> HEDEIKKLRTSGSMTQNPHEVARVRNLNRIIMGKYEIEPWYFSPYPIELTDEDFIYIDDFTLQYFGSKKQYERYRKKCTLRHPPGNEIYRDDYVSFFEIDGRKQRTWCRNLCLLSKLFLDHKTLYYDVDPFLFYCMTRRDELGHHLVGYFSKEKESADGYNVACILTLPQYQR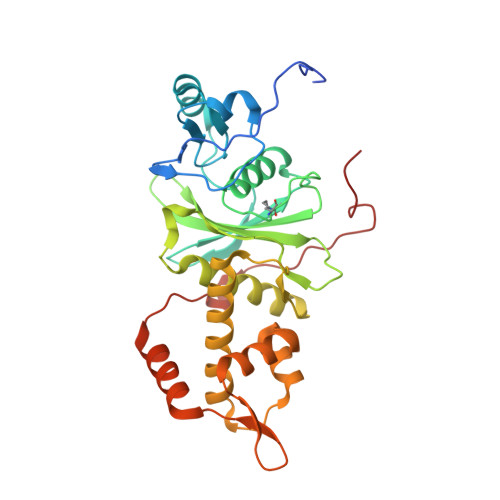MGYGKLLIEFSYELSKKENKVGSPEKPLSDLGLLSYRAYWSDTLITLLVEHQKEITIDEISSMTSMTTTDILHTAKTLNILRYYKGQHIIFLNEDILDRYNRLKAKKRRTIDPNRLIWKPPVFTASQLRFAW Complement factor H (FH), a 155-kDa soluble glycoprotein abundant in human plasma, is an important regulator of the complement system, the chief molecular component of innate immunity. FH is a member of the regulators of complement activation (RCA) family that are characterized by possession of repeating compact domains, known as complement control protein modules (CCPs), sushi domains or short consensus repeats. Human FH binds to, and regulates levels of, the first activation-specific cleavage product of complement component C3, C3b. The four FH amino-terminal CCPs (1–4) perform co-factor and C3bBb decay-accelerating activities, while the two carboxyl-terminal CCPs also bind C3b but additionally bind to GAGs.

In this study we describe the crystal structure of the three carboxyl-terminal CCP modules of human FH (CCPs 18–20) at a resolution of 1.8 Å together with analysis of this region in solution by small angle X-ray scattering (SAXS). While the long axes of CCPs 19 and 20 are approximately aligned, with only a ∼32° tilt relative to one another, the long axis of CCP 18 is strongly tilted, by ∼122° with respect to the long axis of CCP 19, and by ∼151° with respect to CCP 20. The short (three-residue) linker between CCPs 19 and 20 (i.e. between the last cysteine of CCP 19 and the first of CCP 20) along with numerous inter-modular contacts imposes an approximately linear rod-like structure on this (GAG/C3b-binding) part of the molecule; the longer (six-residue) 18–19 linker permits a sharp kink to form in the molecule, also stabilized by inter-modular and module-to-linker interactions, but with a smaller inter-modular interface than observed between modules 19 and 20. Atomic distances consistent with hydrogen bond formation are observed between Gln1101 (CCP 18)-Gln1156 (CCP 19); Lys1103 (linker)-Asn1154 (CCP 19); and Lys1103 (linker)-Gln1156 (CCP 19). Furthermore, the surface area buried between CCPs 18 and 19 is only ∼400 Å, compared to almost ∼700 Å for CCPs 19 and 20. Interestingly, though, the experimentally derived scattering curves did not fit well to data back-calculated from the ‘J’-shaped crystal structure (discrepancy χ = 2.4); nor did ab initio low-resolution shape envelopes generated using the program DAMMIF demonstrate the same acute angle between CCPs 18 and 19. The SAXS data were fit well by an ensemble in which the 19–20 linker was fixed (χ = 1.3), but were fit poorly by the ensemble in which the 18–19 linker was fixed (χ = 2.4). Taking these data together, it appears that modules 19 and 20 are rigidly aligned such that their rod-like conformation is independent of the addition of CCP 18 or the presence of ligands.

> AGTSCVNPPTVQNAYIVSRQMSKYPSGERVRYQCRSPYEMFGDEEVMCLNGNWTEPPQCKDSTGKCGPPPPIDNGDITSFPLSVYAPASSVEYQCQNLYQLEGNKRITCRNGQWSEPPKCLHPCVISREIMENYNIALRWTAKQKLYSRTGESVEFVCKRGYRLSSRSHTLRTTCWDGKLEYPTCAKR> GSHMAATAAEAVASGSGEPREEAGALGPAWDESQLRSYSFPTRPIPRLSQSDPRAEELIENEEPVVLTDTNLVYPALKWDLEYLQENIGNGDFSVYSASTHKFLYYDEKKMANFQNFKPRSNREEMKFHEFVEKLQDIQQRGGEERLYLQQTLNDTVGRKIVMDFLGFNWNWINKQQGKRGW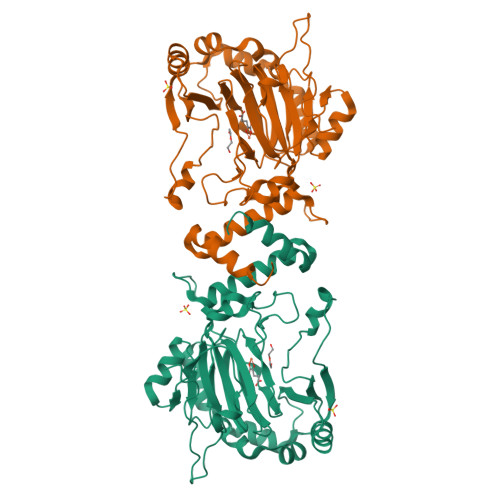GQLTSNLLLIGMEGNVTPAHYEEQQNFFAQIKGYKRCILFPPDQFECLYPYPVHHPCDRQSQVDFDNPDYERFPNFQNVVGYETVVGPGDVLYIPMYWWHHIESLLNGGITITVNFWYKGAPTPKRIEYPLKAHQKVAIMRNIEKMLGEALGNPQEVGPLLNTMIKGRYN(2~{S})-1-(4-fluorophenyl)sulfonyl-~{N}-(2-methyl-5,6-dihydro-4~{H}-cyclopenta[c]pyrazol-3-yl)pyrrolidine-2-carboxamide 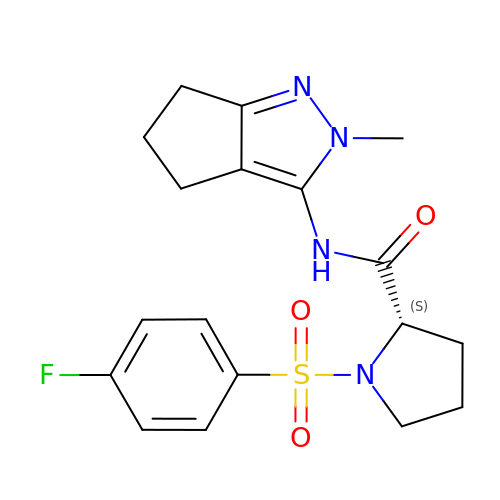| C18 H21 F N4 O3 S | ZYGWHQCDHVLXGI-INIZCTEOSA-N>MKIATLNKGKETKYFNGYPLIEEEDIYSQDHLKEGDIFQIVTDKSQYVATAYVGRQHKGLGWVLTYDKAQEINTAFFVKLFNTALAERDYYFNIDGTNAFRLFNAEGDGVGGLTIDNYDGHLLIQWYSKGIYKFKYAILEAVRKVFDYKSIYEKVRFKDSEYSGGFVEGDAPEFPIVIEENFTFYNVDLEDGLMTGIFLDQKEVRKKLRGQYAKERHVLNLFSYTGAFSVIAASEASSTTSVDLANRSRSLTEENFGLNAIDPKSQYIYVMDTFDFYKYAARHGHSYDTIVIDPPSFARNKKRTFSVQKDYDKLINGALNIL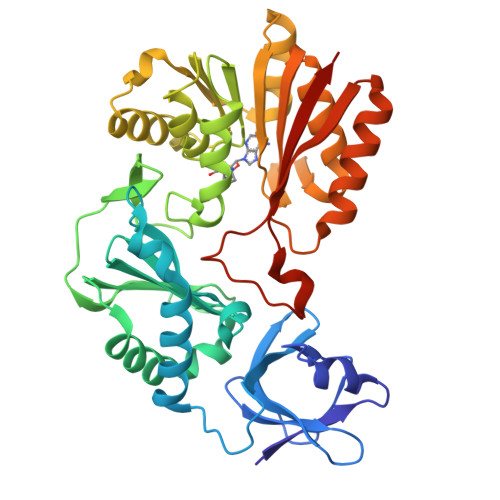SSEGTLLLCTNASVYPLKQFKNTIKKTLEESGVDYELTEVMGLPKDFKTHPHYKPSKYLKAVFVNIRHLEHHHHHH[4x]> PISPIETVPVKLKPGMDGPKVKQWPLTEEKIKALVEICTEMEKEGKISKIGPENPYNTPVFAIKKKD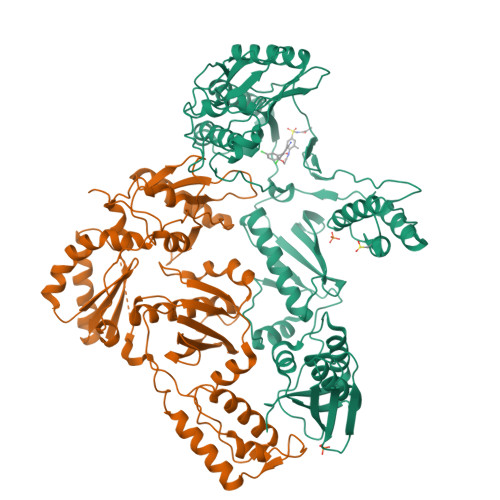STKWRKLVDFRELNKRTQDFWEVQLGIPHPAGIKKKKSVTVLDVGDAYFSVPLDEDFRKYTAFTIPSINNETPGIRYQYNVLPQGWKGSPAIFQSSMTKILEPFRKQNPDIVIYQYMDDLYVGSDLEIGQHRTKIEELRQHLLRWGLTTPDKKHQKEPPFLWMGYELHPDKWTVQPIVLPEKDSWTVNDIQKLVGKLNWASQIYPGIKVRQLCKLLRGTKALTEVIPLTEEAELELAENREILKEPVHGVYYDPSKDLIAEIQKQGQGQWTYQIYQEPFKNLKTGKYARMRGAHTNDVKQLTEAVQKITTESIVIWGKTPKFKLPIQKETWETWWTEYWQATWIPEWEFVNTPPLVKLWYQLEKEPIVGAETFYVDGAANRETKLGKAGYVTNRGRQKVVTLTDTTNQKTELQAIYLALQDSGLEVNIVTDSQYALGIIQAQPDQSESELVNQIIEQLIKKEKVYLAWVPAHKGIGGNEQVDKLVSAGIRKVL;> PISPIETVPVKLKPGMDGPKVKQWPLTEEKIKALVEICTEMEKEGKISKIGPENPYNTPVFAIKKKDSTKWRKLVDFRELNKRTQDFWEVQLGIPHPAGLKKKKSVTVLDVGDAYFSVPLDEDFRKYTAFTIPSINNETPGIRYQYNVLPQGWKGSPAIFQSSMTKILEPFRKQNPDIVIYQYMDDLYVGSDLEIGQHRTKIEELRQHLLRWGLTTPDKKHQKEPPFLWMGYELHPDKWTVQPIVLPEKDSWTVNDIQKLVGKLNWASQIYPGIKVRQLCKLLRGTKALTEVIPLTEEAELELAENREILKEPVHGVYYDPSKDLIAEIQKQGQGQWTYQIYQEPFKNLKTGKYARMRGAHTNDVKQLTEAVQKITTESIVIWGKTPKFKLPIQKETWETWWTEYWQATWIPEWEFVNTPPLVKLWYQLEKEPIVGAETF> MGSSHHHHHHSQDPMSLLARLAPHLPYIRRYARALTG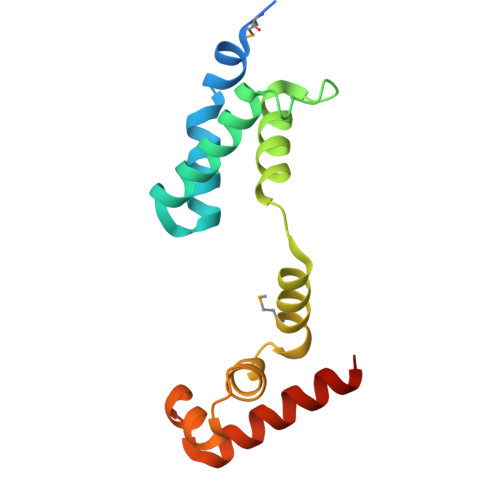DQATGDHYVRVALEALAAGELVLDANLSPRVALYRVFHAIWLSSAGDDAAQRLMRIAPRSRQAFLLTALEGFTPTEAAQILDCDFGEVERLIGDAQAEIDAELAT>DGGEYLRPEDLKELGDDSLPSSQFLDGMNYLRYSLEGGRSLVPRGSGSRNGITPLHVASKRGNTNMVKLLLDRGGQIDAKTRDGLTPLHCAARSGHDQVVELLLERGAPLLARTKNGLSPLHMAAQGDHVECVKHLLQHKAPVDDVTLDYLTALHVAAHCGHYRVTKLLLDKRANPNARALNGFTPLHIACKKNRIKVMELLVKYGASIQAITESGLTPIHVAAFMGHLNIVLLLLQNGASPDVTNIRGETALHMAARAGQVEVVRCLKVVTEEVTT[2x]

Ankyrins are a widely expressed scaffold protein family, which mainly function to link great varieties of functionally related but structurally diverse integral membrane proteins to the spectrin-based cytoskeletons. Each ankyrin contains an N-terminal membrane binding domain (MBD), which is composed of 24 ANK repeats and responsible for binding to diverse membrane targets. Following the MBD is an unstructured linker region of ~130 amino acid residues, followed sequentially by a ZU5-ZU5-UPA supramodule responsible for spectrin binding (SBD), a death domain (DD), and an intrinsically disordered C-terminal tail (CT) with varying lengths. We identified three distinct autoinhibitory segments from the intrinsically disordered linker and CT regions of AnkB, and elucidated the inhibition mechanism of these segments by detailed biochemical and structural investigations.

First, we mapped the minimal regions of AI-b and the corresponding repeats from MBD responsible for the interaction. Using the scheme described in Figure 2E as the assay, we mapped AI-b to a 32-aa fragment (aa 865–896) from the linker. Using a similar approach combined with truncations of various repeats, we mapped the AI-b binding regions to R6-14 of MBD. We determined the crystal structure of AnkB repeats 8–14 fused to the C-terminus of AnkB_AI-b (aa 857–896) at 2.35 Å resolution. The AI-b peptide binds to the inner groove formed by repeats 10–13, covering a large portion of the target binding ‘site-3’ (repeats 11–14) and a small portion of ‘site-2’ (repeats 7–10) that were defined in our previous study. The structure is also consistent with our biochemical data that the autoinhibitory interaction mediated by AI-b partially inhibits the binding of Nav1.2 and NF186 to MBD, as both targets use the ‘site-3’ of MBD as one of the binding sites. The electron densities of the MBD_R8-14 bound AI-b only allowed us to trace residues spanning Gly883-Glu892. Although residues Glu865-Asp882 could not be traced in the crystal structure, this segment also directly participates in binding to MBD_R8-14, as deletion of residues from 865 to 873 significantly weakened AI-b’s binding to AnkB_MBD. The structure of the MBD_R8-14/AI-b complex reveals their binding details: Tyr886 forms a hydrogen bond with His374 and hydrophobic interactions with Phe399 and Ile404; Met884 inserts into a hydrophobic pocket formed by Lys407, Val437, Phe440 and Met441; and Arg888 forms a number of hydrogen bonds with the sidechain of Tyr365 and backbone of Leu363 as well as charge-charge interaction with Asp364. ITC results showed that single point substitution of Tyr886 from AI-b with Ala significantly decreased its binding to MBD, and Met884Ala, Tyr886Ala double mutations totally abolished the AI-b’s autoinhibition.> MKTRLTNNVDRQSALYGSSGGTAAQRYEQLRVDRNSPLKRA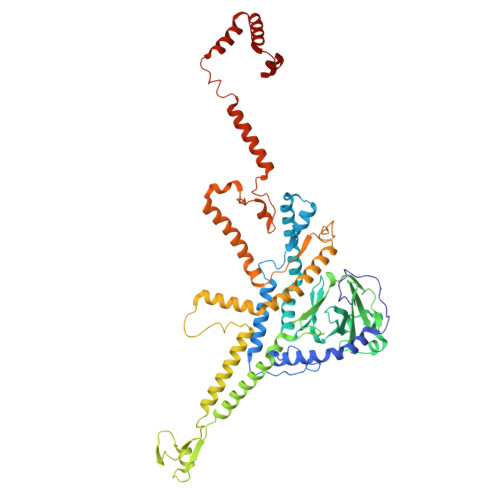RDCSKVTIPGLIEDENYGDAGRLDTPYQSSGARGVGHMTSKLAVTLFPTNEHFFKLEIDSLAILASDQNPEMITEFDSALVKVEQAVMRMFETIGGRAAMHEALKHLLVGGNVLLYVSDEGIKVIHLDSYVLCRDPMGNVTEIVVEEEIFKDALPEEYLDEEDDDDDDMGKKMVKIYTCIKFMDDQCHWYQEIKGKEVPGTHGKCAADVAPWIALRQDRVDSEMYGRSYVEQYYGDLLALENLYKAILEASASLSKVLFLCNPNGTTRPRTLSQASNGSIVQGNAADVTVLQAAGKSQDLQIANQTIERIENRLAFAFMLNTAIQRPGERVTAEEIRYMAQELDAGISGLYSILSRELQLPLVRRLIHILRRKRKLPDFPRSEVTGEPLIKEKAVTGIEAIGRGDDRNKLIDFITTANQALGPQAMTQFLNVEEALRRLAASGSIDTTNLVKTKAQLQQEAAAQAEAEQQAQQQQLLETGIKSPAMAQAVKNFQGADPERAAQALSAITSETGGIDADQLTEAV> SRRVTRAVRPTKRIEFTEADGDTEGKSVFQLEKETDKETFKIRDDNPWVTVETNGAVRVKKKWDYEELGPEKTIDFWVIITNMGHNAGIKYTDNQRVIILVKDVNDEPPYFINRPLPMQAVVQLNAPPNTPVFTLQARDPDTDHNIHYFIVRDRTGGRFEVDERSG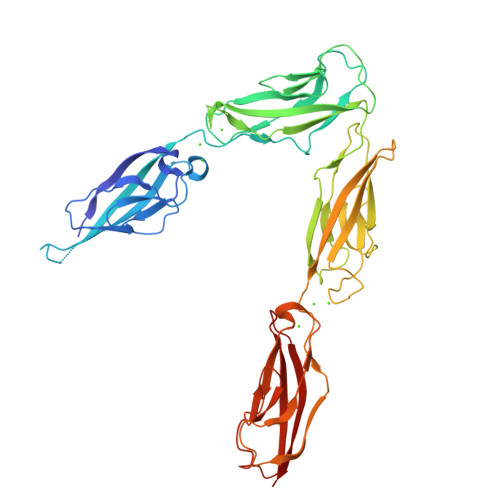VVRTRGTDLFQLDMEYVLYVKAEDQNGKVDDRRFQSTPEERLSIVGGKRAPQFYMPSYEAEIPENQKKDSDIISIKAKSFADREIRYTLKAQGQGAGTFNIGPTSGIVKLAKELDFEDLRQPHVYSLIVTATEDSGGFSTSVDLTIRVTDVNDNAPKFELPDYQAHNVDEDIPLGTSILRVKAMDSDSGSNAEIEYLVSDDHFAVDSNGIIVNNKQLDADNNNAYYEFIVTAKDKGEPPKSGVATVRVYTKNK> MNYKELEKMLDVIFENSEIKEIDLFFDPEVEISKQEFEDLVKNADPL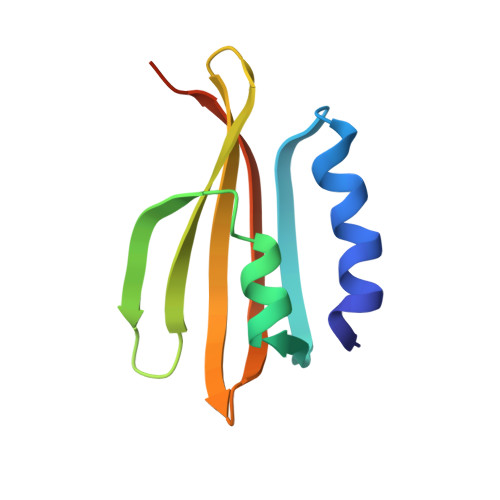QKVVGDNYITETFEWWEFENQYLEFELDYYVKDEKIFVLEMHFWRKIRKLEHHHHHH> MDSNTVSSFQVDCFLWHVRKRFADQELGDAPFLDRLRADQASLRGRGNTLGLDIETATRAGKQIVERILEGESDKALKMPASRYLTDMTLEEMSRDWFMLMPKQKVAGSLCIKMDQAIMDKTIILKANFSVIFDRLETLILLRAFTEEGAIVGEISPLPSLPGHTGEDVKNAIGVLIGGLEWNDNTVRVTETIQRFAW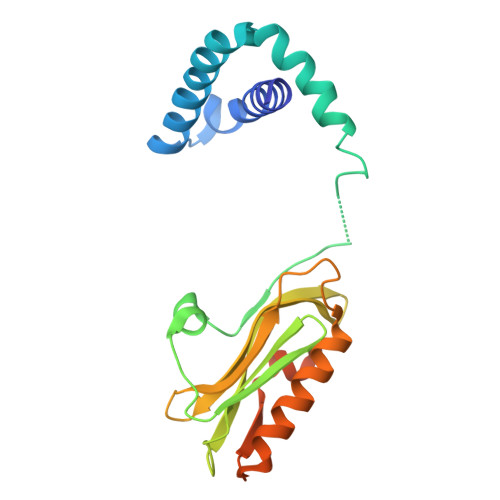RNSDEDGRLPLPPNQKR>AHSIRVDGDIILGGLFPVHAKGERGVPCGELKKEKGIHRLEAM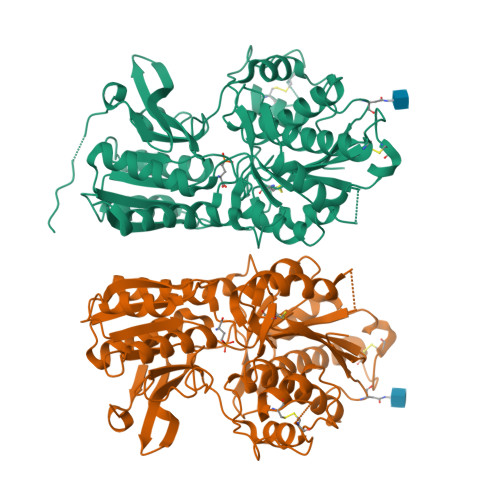LYAIDQINKDPDLLSNITLGVRILDTCSRDTYALEQSLTFVQALIEKDASDVKCANGDPPIFTKPDKISGVIGAAASSVSIMVANILRLFKIPQISYASTAPELSDNTRYDFFSRVVPPDSYQAQAMVDIVTALGWNYVSTLASEGNYGESGVEAFTQISREIGGVSIAQSQKIPREPRPGEFEKIIKRLLETPNARAVIMFANEDDIRRILEAAKKLNQSGHFLWIGSDSWGSKIAPVYQQEEIAEGAVTILPKRASIDGFDRYFRSRTLANNRRNVWFAEFWEENFGCKLGSHGKRNSHIKKCTGLERIARDSSYEQEGKVQFVIDAVYSMAYALHNMHKDLCPGYIGLCPRMSTIDGKELLGYIRAVNFNGSAGTPVTFNENGDAPGRYDIFQYQITNKSTEYKVIGHWTNQLHLKVEDMQWAHREHTHPASE[2x]>VFGSRNDRTLRRMRKVVNIINAMEPEMEKLSDEELKGKTAEFRARLEKGEVLENLIPEAFAVVREASKRVFGMRHFDVQLLGGMVLNERCIAEMRTGEGKTLTATLPAYLNALTGKGVHVVTVNDYLAQRDAENNRPLFEFLGLTVGINLPGMPAPAKREAYAADITYGTNNEYGFDYLRDNMAFSPEERVQRKLHYALVDEVDSILIDEARTPLIISGPAEDSSEMYKRVNKIIPHLIRQEKEDSETFQGEGHFSVDEKSRQVNLTERGLVLIEELLVKEGIMDEGESLYSPANIMLMHHVTAALRAHALFTRDVDYIVKDGEVIIVDEHTGRTMQGRRWSDGLHQAVEAKEGVQIQNENQTLASITFQNYFRLYEKLAGMTGTADTEAFEFSSIYKLDTVVVPTNRPMIRKDLPDLVYMTEAEKIQAIIEDIKERTAKGQPVLVGTISIEKSELVSNELTKAGIKHNVLNAKFHANEAAIVAQAGYPAAVTIATNMAGRGTDIVLGGSWQAE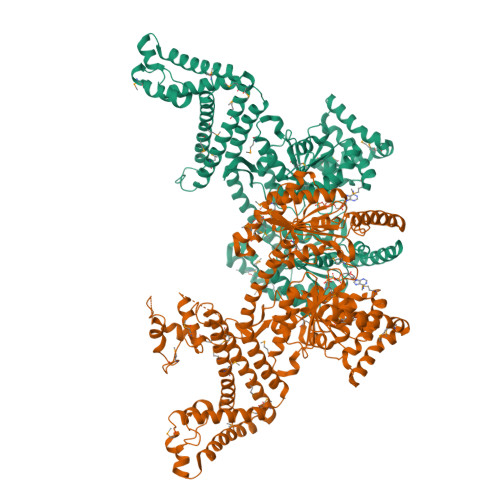VAALENPTAEQIEKIKADWQVRHDAVLEAGGLHIIGTERHESRRIDNQLRGRSGRQGDAGSSRFYLSMEDALMRIFASDRVSGMMRKLGMKPGEAIEHPWVTKAIANAQRKVESRNFDIRKQLLEYDDVANDQRRAIYSQRNELLDVSDVSETINSIREDVFKATIDAYIPPQSLEEMWDIPGLQERLKNDFDLDLPIAEWLDKEPELHEETLRERILAQSIEVYQRKEEVVGAEMMRHFEKGVMLQTLDSLWKEHLAAMDYLRQGIHLRGYAQKDPKQEYKRESFSMFAAMLESLKYEVISTLSKVQVRMPEEVEELEQQRRMEAERLAQMQQLSHQD[2x]>[2x]TNRDIQFTSFNGKDYPLCFLDEKTPLLFQWFERNPARFGKNDIPIINTEKNPYLNNIIKAATIEKERLIGIFVDGDFFPGQKDAFSKLEYDYENIKVIYRNDIDFSMYDKKLSEIYMENISKQESMPEEKRDCHLL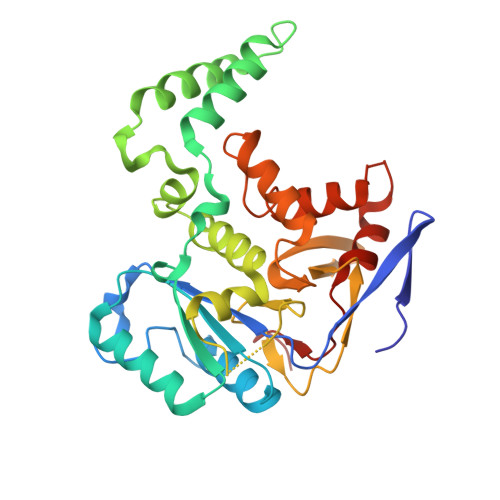QLLKKELSDIQEGNDSLIKSYLLDKGHGWADFYRNMAMLKAGQLFLEADKVGCYDLSTNSGCIYLDADMIITEKLGGIYIPDGIAVHVERIDGRASMENGIIAVDRNNHPALLAGLEIMHTKFDADPYSDGVCNGIRKHFNYSLNEDYNSFCDFIEFKHDNIIMNTSQ>VNGTLMQYFEWYTPNDGQHWKRLQNDAEHLSDIGITAVWIPPAYKGLSQSDNGYGPYDLYDLGEFQQKGTVRTKYGTKSEL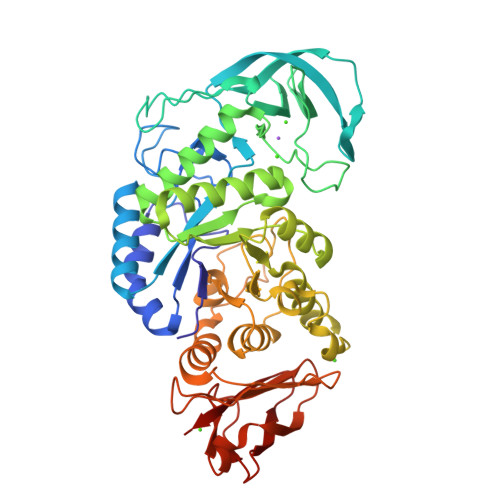QDAIGSLHSRNVQVYGDVVLNHKAGADATEDVTAVEVNPANRNQETSEEYQIKAWTDFRFPGRGNTYSDFKWHWYHFDGADWDESRKISRIFKFRGEGKAWDWEVSSENGNYDYLMYADVDYDHPDVVAETKKWGIWYANELSLDGFRIDAAKHIKFSFLRDWVQAVRQATGKEMFTVAEYWQNNAGKLENYLNKTSFNQSVFDVPLHFNLQAASSQGGGYDMRRLLDGTVVSRHPEKAVTFVENHDTQPGQSLESTVQTWFKPLAYAFILTRESGYPQVFYGDMYGTKGTSPKEIPSLKDNIEPILKARKEYAYGPQHDYIDHPDVIGWTREGDSSAAKSGLAALITDGPGGSKRMYAGLKNAGETWYDITGNRSDTVKIGSDGWGEFHVNDGSVSIYVQK[2x]> G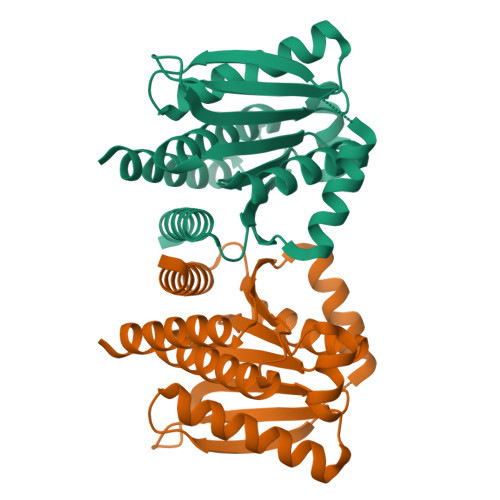AEAAAAAAVTAELRAFRAAGGTVELEDLPVTPETLARAEAALARLPPESVAVETYTVPAPTPEAFLAALEAALARLAAEGLPAILLRVVDADGNLVGSILVAAAGPPAESAAATGRVLTIYVASSPEGLKVARGLAIETRDAGGLALAIGASGAWALAGLAGALALARRLAEAHGAPVRVVTIGDPANPTDAALAAAIRAAYAAALEHHHHHH> MKATQSGQLTAELKRVTRLAAPMATVTIAQYLLPVISVMVAGHNGELQLSGVALATSFTNVTGFSIMYGLVGALETLCGQAYGAKQYEKIGTYTYSAIASNIPICFIISIIWFYIENILISLGQDPDISRIAGSYAFWLIPVLFAQAIVIPLTRFLLTQGLVLPLLYTAVTTLLFHVFVCWVFVLVFVLGSNGPAMATSVSFWFYAVILSCYVRFSSSCEKTRGFVSEDFVSCVKQFFQYGVPSAAMICLEWWLFELLILCSGLLSNPKLETSVLSICLTTETLHYVISSGVAAAVSTRVSNNLGAGNPQVARVSVLAGLCLWLVESAFFSILLFTFRNIIGYAFSNSKEVVDYVADLSPLLCLSFILDGFTAVLNGVARGSGWQHIGAWNNIFSYYLVGAPVGVYLAFRHDLNGKGLWCG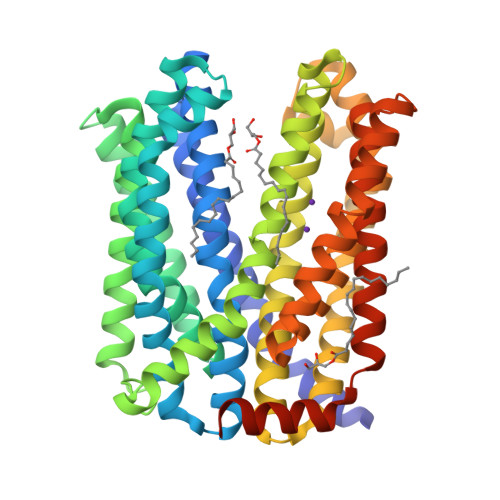VVIGSTVQATVLAIVTASMNWKEQAEKARKRIVSTENELAEFPGENLYFQ> MRGSHHHHHHGMASVFADSLFSDRFNRI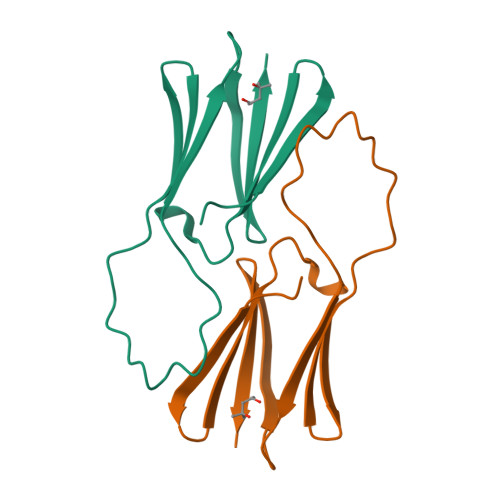DRLFSQLTGDTPVAATPAYDLQKRDANNYLLTVSVPGWKEEELEIETVGGNLNITGKHTEETVEDQTHWIYRGIRKADFQLSFSLPEHAKVNNAKLEQGLLLVEIYQEIPESEKPKKIAIES> MSANNTAKNMHPETRAVGSETSSLQASQDEFENLVRNVDVKSRIMDQYADWKGVRYRLGGSTKKGIDCSGFV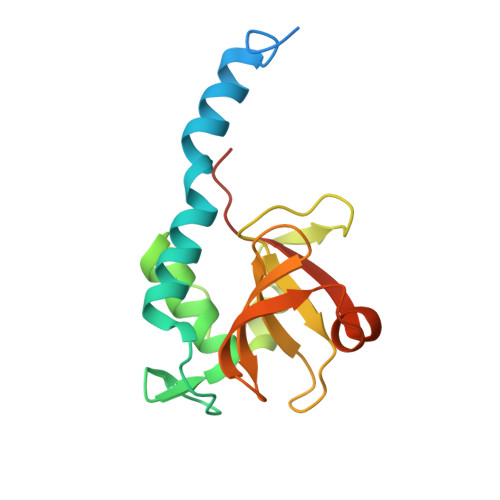QRTFREQFGLELPRSTYEQQEMGKSVSRSNLRTGDLVLFRAGSTGRHVGIYIGNNQFVHASTSSGVIISSMNEPYWKKRYNEARRVLSRSHHHHHH>[5x]MEFLMSKHEADAPH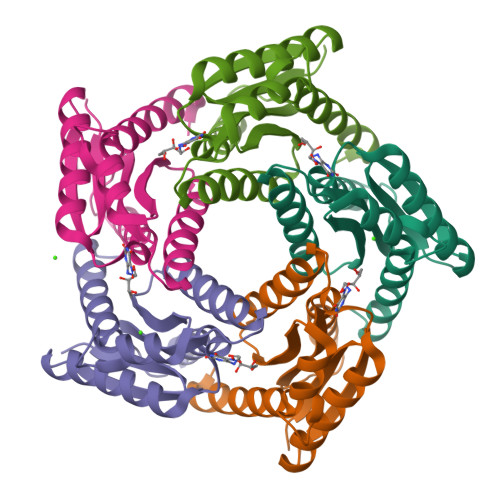LLIVEARFYDDLADALLDGAKAALDEAGATYDVVTVPGALEIPATISFALDGADNGGTEYDGFVALGTVIRGETYHFDIVSNESCRALTDLSVEESIAIGNGILTVENEEQAWVRARREDKDKGGFAARAALTMIGLRKKFGA>MEIIRSNFKSNLHKVYQAIEEADFFAIDGEFSGISDGPSVSALTNGFDTPEERYQKLKKHSMDFLLFQFGLCTFKYDYTDSKYITKSFNFYVFPKPFNRSSPDVKFVCQSSSIDFLASQGFDFNKVFRNGIPYLNQEEERQLREQYDEKRSQANGAGALSYVSPNTSKCPVTIPEDQK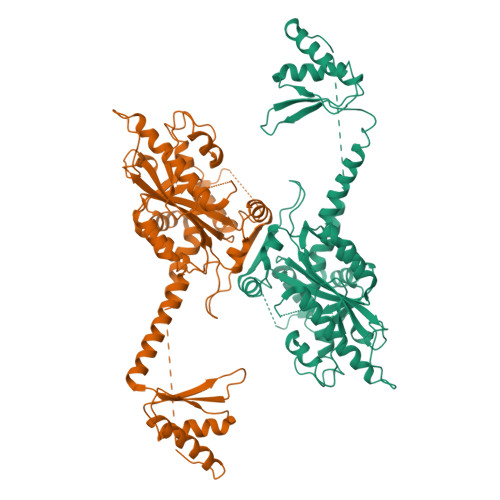KFIDQVVEKIEDLLQSEENKNLDLEPCTGFQRKLIYQTLSWKYPKGIHVETLETEKKERYIVISKVDEEERKRREQQKHAKEQEELNDAVGFSRVIHAIANSGKLVIGHNMLLDVMHTVHQFYCPLPADLSEFKEMTTCVFPRLLDTKLMASTQPFKDIINNTSLAELEKRLKETPFNPPKVESAEGFPSYDTASEQLHEAGYDAYITGLCFISMANYLGSFLSPPKIHVSARSKLIEPFFNKLFLMRVMDI[4x]>MKGFAMLSIGKVGWIEKEKPAPGPFDAIVRPLAVAPCTSDIHTVFEGAIGERHNMILGHEAVGEVVEVGSEVKDFKPGDRVVVPAITPDWRTSEVQRGYHQHSGGMLAGWKFSNVKDGVFGEFFHVNDADMNLAHLPKEI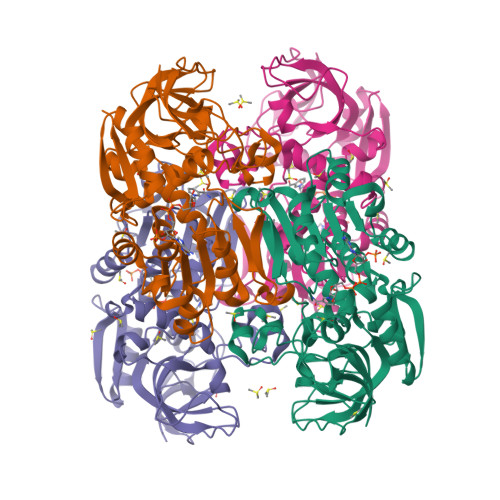PLEAAVMIPDMMTTGFHGAELADIELGATVAVLGIGPVGLMAVAGAKLRGAGRIIAVGSRPVCVDAAKYYGATDIVNYKDGPIESQIMNLTEGKGVDAAIIAGGNADIMATAVKIVKPGGTIANVNYFGEGEVLPVPRLEWGCGMAHKTIKGGLAPGGRLRMERLIDLVFYKRVDPSKLVTHVFRGFDNIEKAFMLMKDKPKDLIKPVVILA[4x]> CGCGAAAA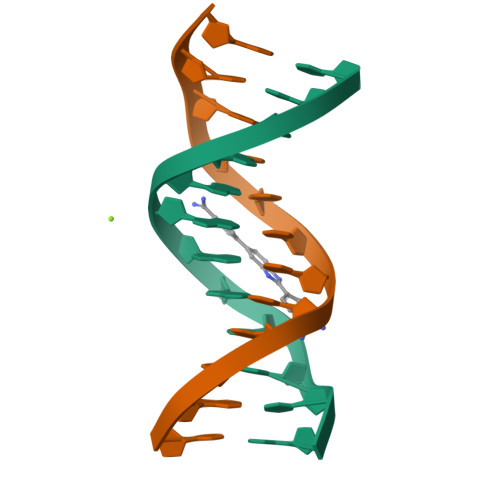CGCG;> CGCGTTTTCGCG> LVTISSTSAASLPTMPPSGYDQVRNGVPRGQVVNISYFSTATNSTRPARVYL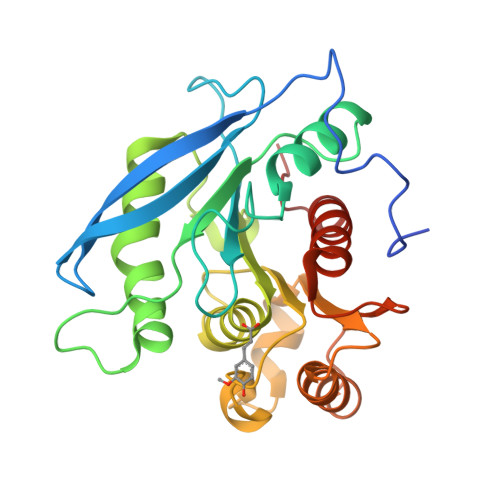PPGYSKDKKYSVLYLLHGIGGSENDWFEGGGRANVIADNLIAEGKIKPLIIVTPNTNAAGPGIADGYENFTKDLLNSLIPYIESNYSVYTDREHRAIAGLAMGGGQSFNIGLTNLDKFAYIGPISAAPNTYPNERLFPDGGKAAREKLKLLFIACGTNDSLIGFGQRVHEYCVANNINHVYWLIQGGGHDFNVWKPGLWNFLQMADEAGLTRDGNT> MADNEKLDNQRLKNFKNKGRDLETMRRQRNEVVVELRKNKRDEHLLKRRNVPHEDICEDSDIDGDYRVQNTSLEAIVQNASSDNQGIQLSAVQAARKLLSSDRNPPIDDLIKSGILPILVHCLERDDNPSLQFEAAWALTNIASGTSEQTQAVVQSNAVPLFLRLLHSPHQNVCEQAVWALGNIIGDGPQCRDYVISLGVVKPLLSFISPSIPITFLRNVTWVMVNLCRHKDPPPPMETIQEILPALCVLIHHTDVNILVDTVWALSYLTDAGNEQIQMVIDSGIVPHLVPLLSHQEVKVQTAALRAVGNIVTGT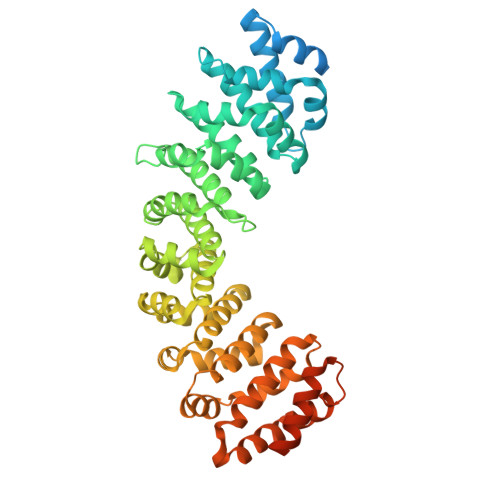DEQTQVVLNCDALSHFPALLTHPKEKINKEAVWFLSNITAGNQQQVQAVIDANLVPMIIHLLDKGDFGTQKEAAWAISNLTISGRKDQVAYLIQQNVIPPFCNLLTVKDAQVVQVVLDGLSNILKMAEDEAETIGNLIEECGGLEKIEQLQNHENEDIYKLAYEIIDQFFSSDDIDEDPSLVPEAIQGGTFGFNSSANVPTEGFQF>METVAAIKTLIQQLAQSTDQFGRAEINDALRELQYSLETPFDTVMRMSLDTCQVAVARIGSDLGLFKHLSQCASPQSAEELADHLGCGRELMSRLLRYMASVRMVQQTDDIKYISSNITQTLAVPGLEAGMRHAFENLWPVLMALPDFLAERKYPDIVDAKDTAFQKAFNTDQDCFHWLATQPTRIANFKVLLTDERTPNFLSTFPLEKELGSWSAEPEKALFVDIGGGMGHACIRLREKYPNQPGRVILQDLPPVLQAAQATLPLSGIESMPHNFHTPQPVQGAKFYFLRLILRDFPDHQALEILQNIVPAMDAESRIVIDDGVPPEKGARWAETGTDICIMSALGSKERTQRQWEELAAKAGLQLQALYQYTWPVVNAAMVFSLQ[2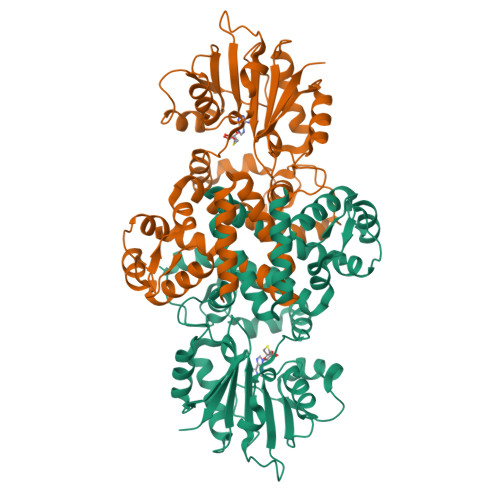x]>MGKIVEIHPTTRHEGHTKLVLKVDDEGIVEKGAYLSVTPVRGFEKFLVGKPAEFAPIAVSRFCGICPVAHATSAVEAIEDACDITPPKDGLLLRELCGIGNKMHSHPLHQFLISPDYVPKDDSNEFIKRVQAMRRIGQYIVDAVGGEAIHSPNIKVGGMAKQITESTKAKMYYKCKEYEKLAKEQLEYLIPIFESRTLNDGTELPEKLGYHDFGYIATHPTYGDRTKIDQDKVVEYTPFDVYDKDVAIQSSTTVPTYNGRLMEVGPRARFSKFFDFKEKGAMALHIARAYEISVLVKRAMEILDELNVNGKTMSDEPIVGDGEKLGLGVHEAARGHNTHQAVIDKDGNIVYYNAIVATTWNIPVISKAVEGTHYKFAEHIVRAYDPCISCATHMIIKDYDDKIIGEKILK[2x];>MDPFGKYKTVVSARAADKTILKKCQDGGIVSAAYIYGLENGLLDGVIVADKDDKLQTTPKVATTVDEVLEAAGTKYTVCPTISVIKSAVREYGCEKLGVVGTPCQIIATRKLMKYPIGFRHVPDKLALIVGIFCMENFPYNGMKTIIEEHCGIKMEDVAKTDIGKGKFWVYSKWGDVKSIKLKETHPYEQQSCHVCMDYTAELADISTGSVGSPDGWSTVFIRTAQGEEFFNKMVEAGALEVKPIEEVKPGLGLVEKLSLTKKEKNAKEIEHRKEIGLPVPY[2x];>[2x]MVKIAHIHLCGCTGCLISLADTYEQLLDILNSVELVYALTLVDEKTEIRETDDKILIEREIPDDIDIALVEGSVCLEDEHSMKDVFDARRKSKIVVALGACAATGGITRFCRGGQMSKPVHSSFVPIGDLIKVDLALPGCPPSPEALVNLITAALNGDTEYLEIYAELAKKTEACGCDLLVNVINKSLCMGCGSCAASCPTRAIEMIDGKPNVLKELCIKCGACSLQCPRIRFPKLIEEIE

FRHs catalyze the reversible H2 oxidation coupled to the reduction of coenzyme F420 (8‐hydroxy‐5‐deazaflavin, ΔG°′ = −10 kJ mol−1). The overall reaction requires three components: the large subunit (FRHA) that harbors the [NiFe] center and oxidizes H2, and the small subunit (FRHG), which contains three [4Fe–4S] clusters to transfer electrons to the flavin adenine dinucleotide (FAD) located in the F420‐reducing module (FRHB, harboring an additional [4Fe–4S] cluster). FRHABG dimerizes and forms dodecameric assemblies of about 16 nm in diameter with a spherical shape and a hollow core. Here, by characterizing the native hydrogenase from the marine methanogen Methanothermococcus thermolithotrophicus (belonging to the Methanococcales order), we provided an unprecedented functional understanding of this enzyme via a synergistic approach of biochemistry, X‐ray crystallography, and spectroscopy.

Despite its sequence conservation with the two other structural homologs, we found that the [NiFe]‐containing FRH from M. thermolithotrophicus (MtFRH) exhibits a dynamic equilibrium between a dodecameric and dimeric state in solution, as highlighted by size exclusion chromatography and native polyacrylamide gel electrophoresis (PAGE). It was therefore not surprising to observe several crystalline forms containing either a dodecameric cubic organization (MtFRHcube) or only a single FRH dimer (MtFRHdimer1 −3). In crystallo spectroscopy on hydrogenases was recently established to verify the redox state of the active site in crystal structures and was applied to the MtFRHdimer3 due to the abundance of crystalline material and the attainable crystal size. RR spectroscopy on MtFRH crystals confirmed the presence of oxidized [4Fe–4S] and [2Fe–2S] clusters. The overall intensity of the Fe–S bands and observation of [2Fe–2S]+ specific signals indicate a more oxidized electron transfer (ET) chain in the as‐isolated state compared to MbFRH. Moreover, IR and RR spectroscopy confirmed the presence of the Nia‐S state, previously observed in MbFRH. This state was postulated to be mandatory for the thermodynamically favorable binding of H2 and corroborated the vacant position observed in the crystal structure. IR spectra recorded at different temperatures and exposure to intense illumination did not significantly impact the spectroscopic pattern, excluding temperature‐dependent shifts of the redox state equilibria or the presence of a light‐sensitive species, as observed recently in other hydrogenases. In comparison to known and well‐characterized [NiFe]‐hydrogenases, the crystals turned out to be mostly redox‐inert.> GRNKSSLLFKESEETRTPNC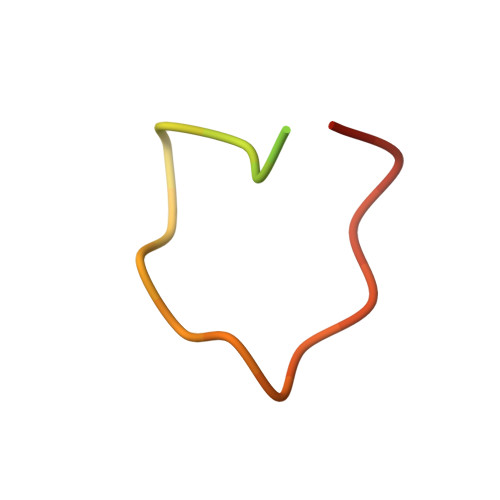NCKYCSHPVLG>MLVLGLNGNFSAADTDVVPQLGEVFFHDSAASLIRDGELVAAVEEERLNRIKKTTKFPLNAVRECLALAGARPEDVDAVGYYFPENHIDTVLNHLYTEYPRAPLRYSRELIRQRLKEGLGWDLPDEKLVYVPHHEAHAYSSYLHSGMDSALVLVLDGRGELHSGTVYRAEGTRLEKLADYPVPKSLGGLYLNATYLLGYGFGDEYKVMGLAPWGNPETYRDTFAKLYTLQDNGEYELHGNIMVPNLVSPLFYAEGFRPRRKGEPFTQAHRDFAAALQETVEKIVLHILEYWAKTSGHSRLCFGGGVAHNSSLNGLILKSGLFDEVFVHPASHDAGAGEGAAYAAAASLGTLERPGKRLLSASLGPALGGREQIRARLADWAPLIDVEFPDDAVETAAGLLAEGQVLGWAYGRSEFG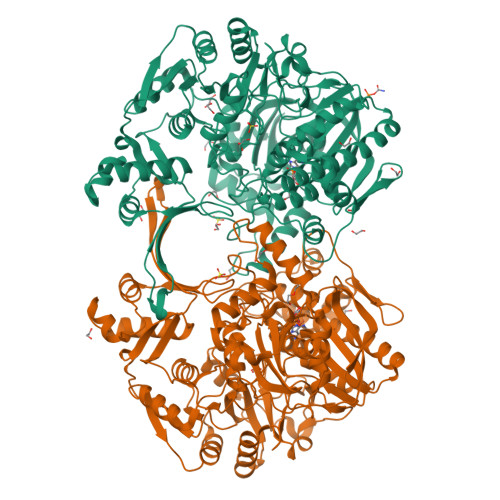PRALGHRSIVADARPEENRTRINAMVKKREGFRPFAPVVTAEAARDYFDLSGADGNHEFMSFVVPVLPERRTELGAVTHVDGTARVQVVSAESGERFHRLVRRFGELTGTPVLLNTSFNNNAEPIVQSLDDVVTSFLTTDLDVLVVEDCLVRGKASPDLGVLVPRFRPVTRLVERRTAGPDASAGAKTHEIHLDYDGGPSAKVSPELYELLGAVDGTTTLGDLAKTVGGLSDALATEVFALWEQRFLTLAPAGDIGPLADDGTRGH[2x]>[2x]SMRKKIFKPEELRQALMPTLEALYRQDPESLPFRQPV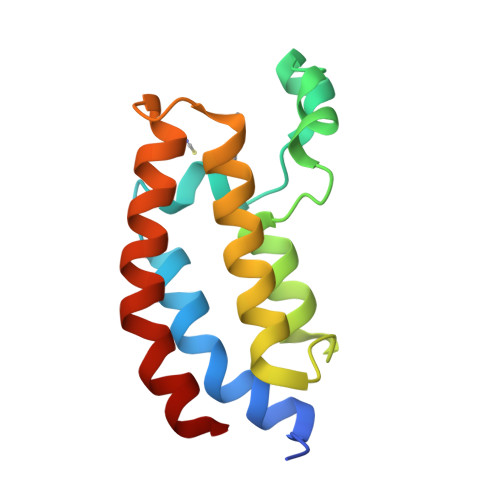DPQLLGIPDYFDIVKNPMDLSTIKRKLDTGQYQEPWQYVDDVWLMFNNAWLYNRKTSRVYKFCSKLAEVFEQEIDPVMQSLG>GPGAGTVGGFIKRQQSKVVQNKVVYYGVGIWRGFMDGYQVHLEIENDIGQPPRLRNVTTNCQSSPWDLSIPIRQWAEDMGVTNNQDYSSKSSRGARYWMHSFRMQGPSKPFGCPVYIIK[2x]

The L protein is a multifunctional enzyme catalyzing genome replication as well as viral transcription. As demonstrated for the influenza virus polymerase complex, the bunyavirus L protein is assumed to bind to cap structures of cellular mRNAs, while an endonuclease cleaves the mRNA some nucleotides downstream of the cap creating a short RNA fragment. This capped RNA fragment is subsequently used to prime viral transcription. Here we present the structure of a small globular domain located in the C-terminal region of RVFV L protein along with the first evidence for a functional cap-binding site within the bunyavirus L protein.

RVFV CBD crystallized as a dimer, which is not fully symmetric, with a buried surface area of ~430 Å2 between the monomers. In solution, the protein appears to be monomeric, as revealed by size-exclusion chromatography (S4 Fig, buffer composition: 50 mM Na-phosphate, pH 6.5, 150 mM NaCl, 10% (w/v) glycerol). The structure of RVFV CBD consists of a β-sheet formed by seven β-strands, an additional β-hairpin as well as a long α-helix. Thus, m7GTP was present in all crystallization setups and additional electron density corresponding to an m7GTP ligand was indeed clearly visible in both chains of the RVFV CBD structure. The m7GTP molecule was bound in a small, mainly hydrophobic pocket between two aromatic amino acid side chains, F1713 and Y1728. The phosphate moiety of the cap structure interacts with R1716 side chain, which is extending from the loop between the first β-strand and the β-hairpin. Further contacts with the m7GTP involve M1782, interacting with the guanine moiety and ribose of the cap-structure, as well as Q1717, interacting with the guanine moiety. Isothermal titration calorimetry (ITC) measurements revealed a KD of ~737 μM of RVFV CBD for m7GTP, which is considerably higher than the KD of 1.5 μM reported for m7GTP binding to influenza virus PB2. In summary, changes of the chemical properties of side chains directly interacting with m7GTP in the RVFV CBD structure mostly result in selective transcription defects in the context of the full-length L protein. The binding site topology of the RVFV L protein cap-binding domain, however, is different from the PB2 cap-binding site: The corresponding essential aromatic residue from the end of the long α-helix (α1) in PB2 (F404) is absent in the RVFV structure.> MNDAAEVALYERLLQLRVLPGASDVHDVRFVFGDDSRCWIEVAMHGDHVIGNSHPALDP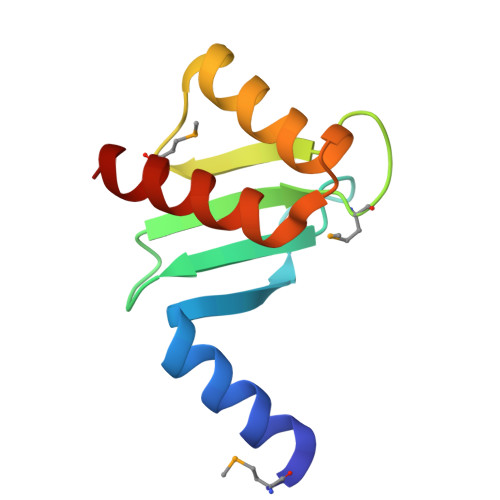KSRATLEHVLTVQGDLAAFLVVARDMLLASL> MSLQQEVDIKTKKLKKLFSKLQAVKAEIHDLQEEHIKERQELEQTQNELTRELKLKHLIIENFIPLEEKNKIMNRSFFDDEEDHWKLHPITRLENQQMMKRPVSAVGYKRPLSQHARMSMMIRPEPRYRAENIMLLELDMPSRTTRDYEGPAISPKVQAALDAALQDEDEIQVDASSFESTASRKPKARPKSGRKSGSSSSSSGN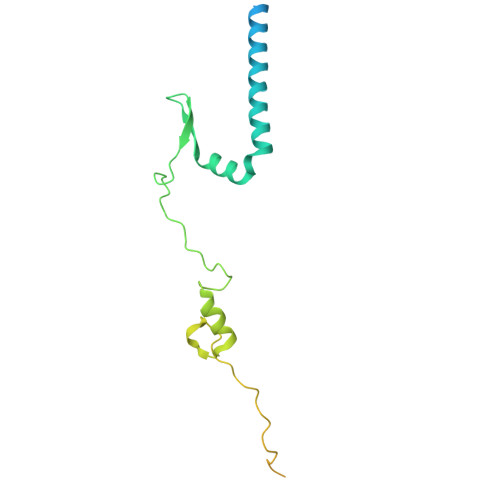PASQFYPQSRGLVPK>[8x]GHMAEINIYQNPGQSLANIYKGFARQCNPGFVFPEAQTIEAWDIPLRLHPEFIPGGDISKADQQYSTLLAQEIANGVTIGFRMVNEKERVCNVE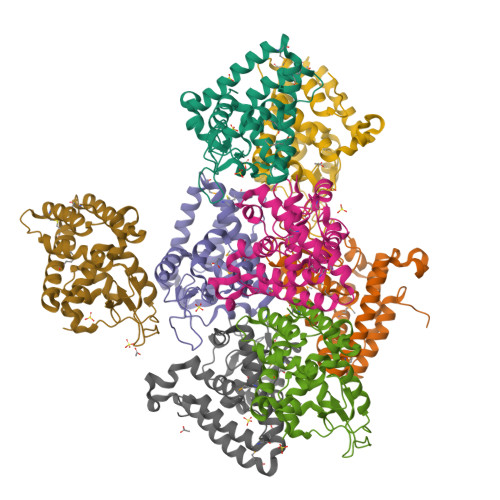ILPLLTSMAQNLDRIKARFGSGYLDRFKGSPNVYPTDVGFSTDASGGISQESGLLVSYGVNLRTLTPGTWQAMTLPEDIKALVGPGVGLRLDAPNFSDVFNTIKSGLRYTTAVTLLLAYFAAIGS> GPLGSGILMAPKTFWVNEGKHAKFRCYVMGKPEPEIEWHWEGRPLLPDRRRLMYRDRDGGFVLKVLYCQAKDRGLYVCAARN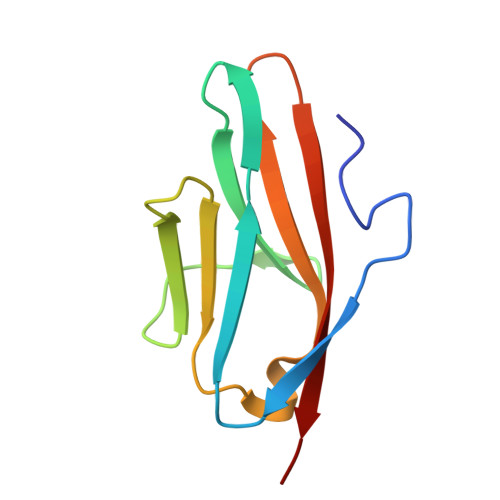SAGQTLSAVQLHVKEP~{N}-[2-[2-[2-[2-[2-[2-[(1-methylquinolin-4-yl)methyl]-1,3-benzothiazol-3-yl]ethanoylamino]ethoxy]ethoxy]ethoxy]ethyl]pentanamide 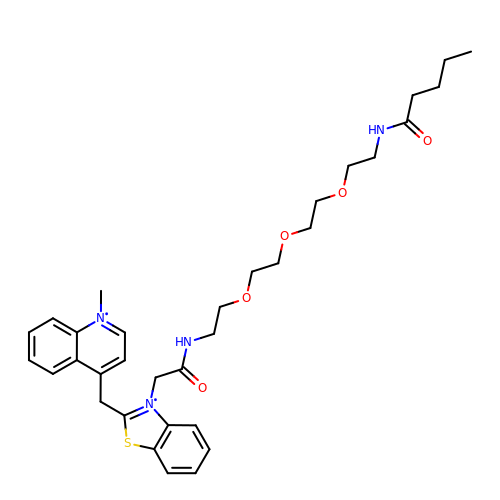| C33 H44 N4 O5 S | HYWIHCYNOZASJE-UHFFFAOYSA-N>[8x]MGSSHHHHHHSSGRENLYFQGMELLKHLSQRQYIDGEWVESANKNTRDIINPYNQEVIFTVSEGTKEDAERAILAARRAFESGEWSQETAETRGKKVRAIADKIKEHREALARLETLDTGKTLEESYADMDDIHNVFMYFAGLADKDGGEMIDSPIPDTESKIVKEP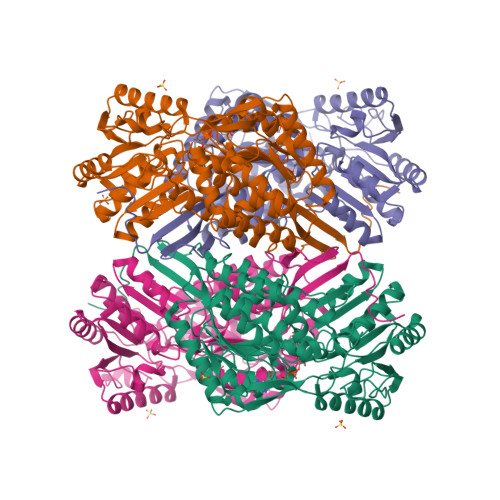VGVVTQITPWNYPLLQASWKIAPALATGCSLVMKPSEITPLTTIRVFELMEEVGFPKGTINLILGAGSEVGDVMSGHKEVDLVSFTGGIETGKHIMKNAANNVTNIALELGGKNPNIIFDDADFELAVDQALNGGYFHAGQVCSAGSRILVQNSIKDKFEQALIDRVKKIKLGNGFDADTEMGPVISTEHRNKIESYMDVAKAEGATIAVGGKRPDRDDLKDGLFFEPTVITNCDTSMRIVQEEVFGPVVTVEGFETEQEAIQLANDSIYGLAGAVFSKDIGKAQRVANKLKLGTVWINDFFPLFAQAPWGGYKQSGIGRELGKEGLEEYLVSKHILTNTNPQLVNWFSK> MGSSHHHHHHSSGAAKGELVGSKVLVRNDRDANRLYSSMYGKPSRRGLQLWPEEALFLCEIGRLEVRSGNVRISPEELMDRFVEEDPRFPVRYAVYADLRRRGWKPKPGRKFGTEFRAFRGEDERIAVKVLQEELDEFTAQDILEWLKLVEGTEFELVVAIVDNDYDLNYYVFSELVLGGGLCAGNGGKELPRAKVFEGGSLVSKDYEDLKRRYFGTE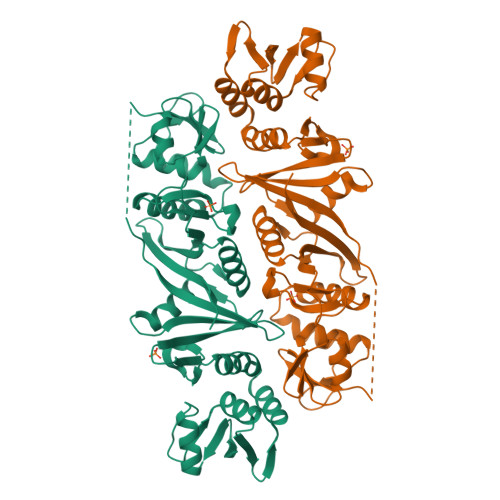HGNVLFLDPFETVYLTEKGEIDPETPEGEPMSVEELLSFFERRRPGFRAGYVVYRDLTERGYVVKSGFKYGGRFRVYEEDPDREHSKYVVRVVEPDTELSTRDVLRATRLAHSVRKDFVLAVVEDVEEPRIEYVMWRWKRL> MGHHHHHHSSPKIEERTYPPQIPAQQELGDFSAYQSVLPEP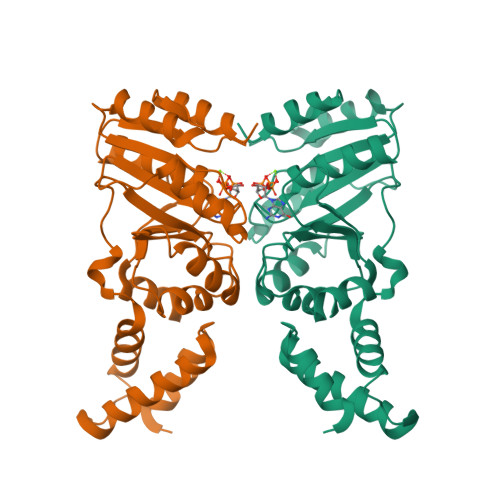LRKAEKLLQETGIKESTKTNTLKKLLRFSVEAGGLTEENVVGKLQEILCDMLPSADKWQEPIHSKYIVLFGSTGAGKTTTLAKLAAISMLEKHKKIAFITTDTYRIAAVEQLKTYAELLQAPLEVCYTKEEFQQAKELFSEYDHVFVDTAGRNFKDPQYIDELKETIPFESSIQSFLVLSATAKYEDMKHIVKRFSSVPVNQYIFTKIDETTSLGSVFNILAESKIGVGFMTNGQNVPEDIQTVSPLGFVRMLCR[6-methyl-5-oxidanyl-4-[(~{E})-2-oxidanylideneundecyliminomethyl]pyridin-3-yl]methyl 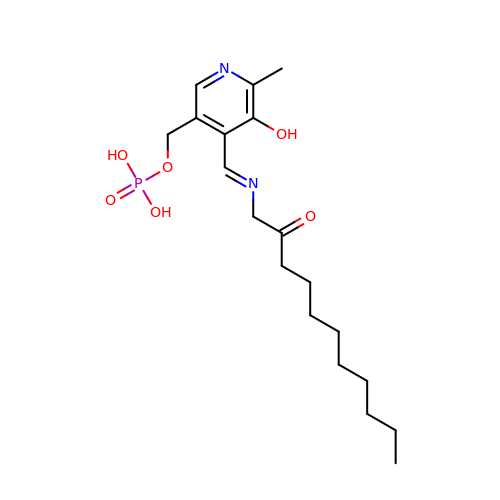dihydrogen phosphate | C19 H31 N2 O6 P | NFGPSQDCIMWBHR-DEDYPNTBSA-N> SSFEGQMAEYPTISIDRFDRENLRARAYFLSHCHKDHMKGLRAPTLKRRLECSLKVYLYCSPVTKELLLTSPKYRFWKKRIISIEIETPTQISLVDEASGEKEEIVVTLLPAGHCPGSVMFLFQGNNGTVLYTGDFRLAQGEAARMELLHSGGRVKDIQSVYLDTTFCDPRFYQIPSREECLSGVLELVRSWITRSPYHVVWLNCKAAYGYEYLFTNLSEELGVQVHVN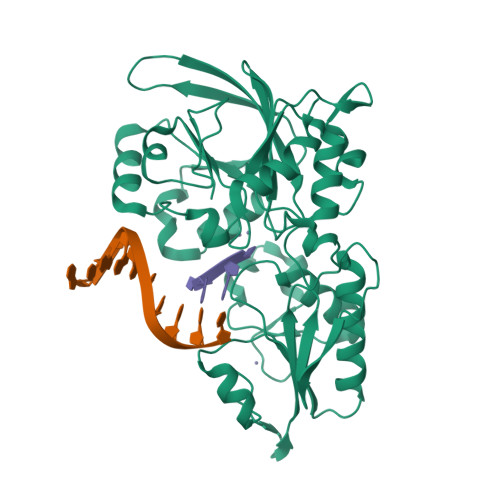KLDMFRNMPEILHHLTTDRNTQIHACRHPKAEEYFQWSKLPCGITSRNRIPLHIISIKPSTMWFGERSRKTNVIVRTGESSYRACFSFHSSYSEIKDFLSYLCPVNAYPNVIPVGTTMDKVVEILKPLCRSSQSTEPKKGENLYFQ>MEKTCIDALPLTMNSSEKQETVCIFGTGDFGRSLGLKMLQCGYSVVFGSRNPQKTTLLPSGAEVLSYSEAAKKSGIIIIAIHREHYDFLTELTEVLNGKILVDISNNLKINQYPESNAEYLAHLVPGAHVVKAFNTISAWALQSGALDASRQVFVCGNDSKAKQRVMDIVRNLGLTPMDQGSLMAAKEIEKYPLQLFPMWRFPFYLSAVLCVFLFFYCVIRDVIYPYVYEKKDNTFRMAISIPNRIFPITALTLLALVYLPGVIAAILQLYRGTKYRRFPDWLDHWMLCRKQLGLVALGFAFLHVLYTLVIPIRYYVRWRLGNLTVTQAILKKENPFSTSSAWLSDSYVALGILGFFLFVLLGITSLPSVSNAVN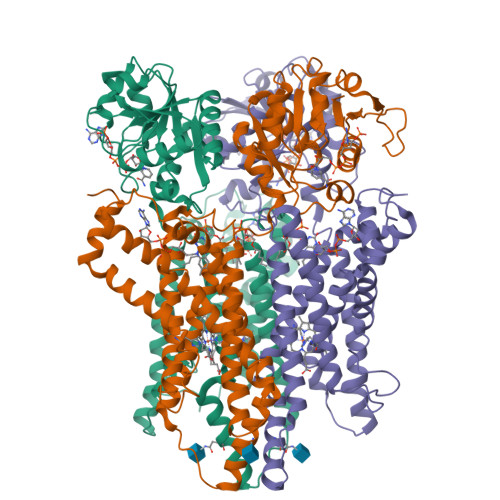WREFRFVQSKLGYLTLILCTAHTLVYGGKRFLSPSNLRWYLPAAYVLGLIIPCTVLVIKFVLIMPCVDNTLTRIRQGWERNSKH[3x]> GHMRKDGFDLDLTYVTDHVIAMSFPSSGRQSLFRNPIGEVSRFFKTKHPDKFRIYNLCSERGYDETKFDNHVYRVMIDDHNVPTLVDLLKFIDDAKVWMTSDPDHVIAIHCKGGKGRTGTLVSSWLLEDGKFDTAKEALEYFGSRRTDFEVGDVFQGVFTASQIRYVGYFEKIKKNYGGQLPPMKKLKVTGVTITAIQGVGRGNGSDLSMQIVSERQEVLLCKFAEGYNCALQYDATDDCVTCEVKNCPVLAGDIKVRFMSTSKSLPRGYDNCPFYFWFNTSL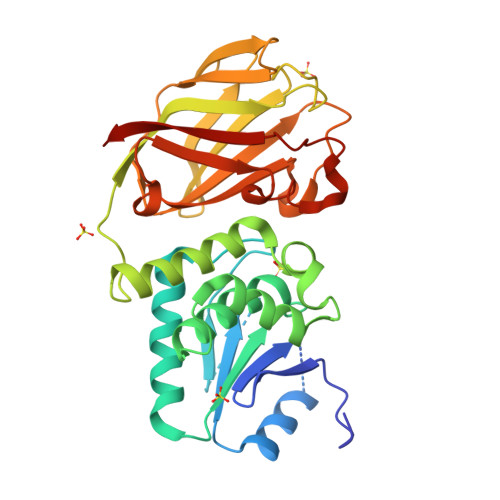VEGDHVTLKREEIDNPHKKKTWKIYRDNFTVKLTFSDAEDI>SITENTSWNKEFSAEAVNGVFVLCKSSSKSCATNDLARASKEYLPASTFKIPNAIIGLETGVIKNEHQVFKWDGKPRAMKQWERDLTLRGAIQVSAVPVFQQIAREVGEVRMQKYLKKFSYGNQNISGGIDKFWLEGQLRISAVNQVEFLESLYLNKLSASKENQLIVKEALVTEAAPEYLVHSKTGWGMGVTPQV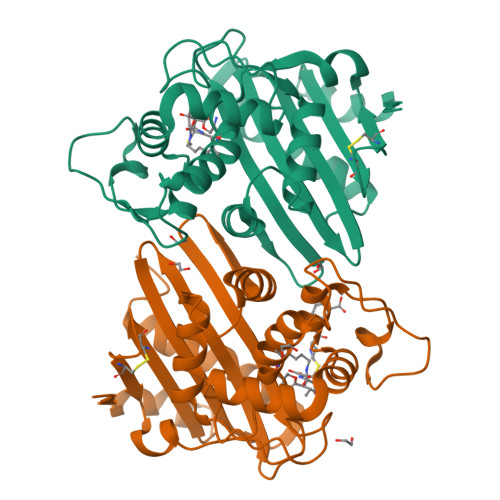GWWVGWVEKETEVYFFAFNMDIDNESKLPLRKSIPTKIMESEGIIGG[4x]> PFATADIAEKMWAENYETTS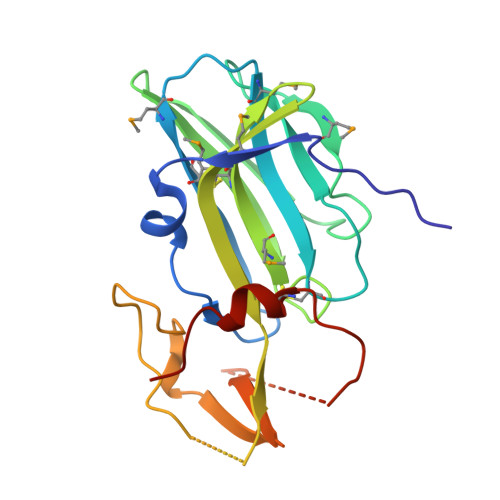PAPVLVAEGEQVTIPCTVMTHSWPMVSIRARFCRSHDGSDELILDAVKGHRLMNGLQYRLPYATWNFSQLHLGQIFSLTFNVSTDTAGMYECVLRNYSHGLIMQRFVILTQLETLSRPDEPCCTPALGRYSLGDQIWSPTPWRLRNHDCGMYRGFQRNYFYIGRADAEDCWKPACPDEEPDRCWTVIQRYRLPGD>MHAALSTEVVHLRQRTEELLRCNEQQAAELETCKEQLFQSNMERKELHNTVMDLRGNIRVFCRIRPPLESEENRMCCTWTYHDESTVELQSIDAQAKSKMGQQIFSFDQVFHPLSSQSDIFEMVSPLIQSALDGYNICIFAYGQSGSGKTYTMDGVPESVGVIPRTVDLLFDSIRGYRNLGWEYEIKATFLEIYNEVLYDLLSNEQKDMEIRMAKNNKNDIYVSNITEETVLDPNHLRHLMHTAKMNRATASTAGNERSSRSHAVTKLELIGRHAEKQEISVGSINLVDLAGSESPKTSTRMTETKNINRSLSELTNVILALLQKQDHIPYRNSKLTHLLMPSLGGNSKTLMFINVSPFQDCFQESVKSLRFAASVNSCKMTK[2x]

Motor proteins of the kinesin family hydrolyze ATP and use the energy released by nucleotide hydrolysis to move along microtubules, performing essential roles in transport, division and other cellular processes. The kinesin-14 motors include Ncd, a motor that plays an essential role in spindle assembly in Drosophila oocytes and functions in the spindle and at the poles in early embryos. Structural studies revealed that Ncd differs from kinesin-1 in that the conserved motor domain or head is joined directly to the α-helical coiled-coil stalk, rather than containing a 'neck linker' between the head and stalk. Ncd, by contrast, is a nonprocessive motor that undergoes a single displacement along a microtubule, then releases from the microtubule, although the motor has been reported to move processively under certain in vitro conditions.

The mutation changes an invariant threonine in the nucleotide-binding motif, GQTGSGKT, to a serine. The NcdT436S mutant has a single amino acid change in the conserved nucleotide-binding P loop that causes the motor to release ADP and hydrolyze ATP faster than wild type, but move more slowly along microtubules in gliding assays, uncoupling ATP hydrolysis from force generation. NcdT436S was crystallized and the structure was solved to 2.8 Å. Remarkably, the model showed a large rotation of the α-helical coiled-coil stalk together with one of the two heads, resulting in asymmetry of the heads, resembling a previously reported crystal structure of NcdN600K. The chain B head shows disrupted interactions with neck residues that are observed in chain A and is positioned to interact with the microtubule, resembling NcdN600K head H2, whereas the chain A head interacts extensively with residues of the neck and has rotated with the stalk, like NcdN600K head H1. The nucleotide-binding cleft is slightly more open in the NcdT436S structure because of the substitution of threonine by the smaller serine. There is a difference in the position of at least one water molecule in the NcdT436S cleft that may explain the more rapid release of ADP by the mutant than wild type. The water molecule forms hydrogen bonds to the S436 hydroxyl group, ADP β-phosphate and G583 amide group, and is present in the head of chain A which rotates with the stalk, but is not visible in the head of chain B. Although density corresponding to the bound ADP and Mg+2 is visible in both NcdT436S heads, the density for the PO4-2 and Mg+2 groups is stronger in the head of chain A than chain B. The NcdT436S structure shows the C-terminal residues of chain B, which contains the head positioned to interact with the microtubule, docked onto the motor core, but the head undocked from the neck. The NcdT436S structure shows that the Ncd C-terminal residues are in the same position as the neck linker of plus-end kinesins, resembling the C-terminal 'neck mimic' of kinesin-14 KCBP.[(2R,3S,4R,5R)-5-(6-amino-9H-purin-9-yl)-4-hydroxy-3-(phosphonooxy)oxolan-2-yl]methyl 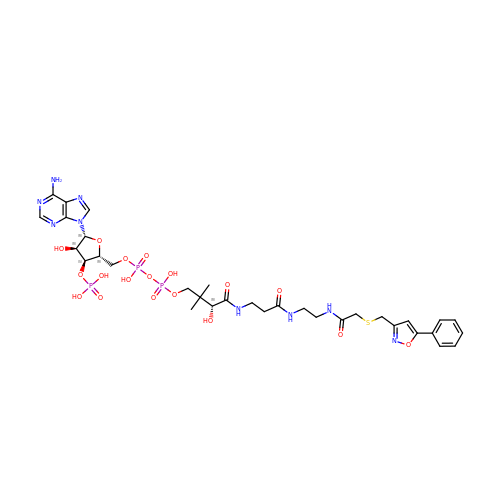(14R)-14-hydroxy-15,15-dimethyl-4,9,13-trioxo-1-(5-phenyl-1,2-oxazol-3-yl)-2-thia-5,8,12-triazahexadecan-16-yl dihydrogen diphosphate | C33 H46 N9 O18 P3 S | YLPJWPUMQHZIRD-GMHMEAMDSA-N>[2x]MKESAAAKFERQHMDSGNSPSSSSTYCNQMMRRRNMTQGRCKPVNTFVHESLVDVQNVCFQEKVTCKNGQGNCYKSNSSMHITDCRLTNGSRYP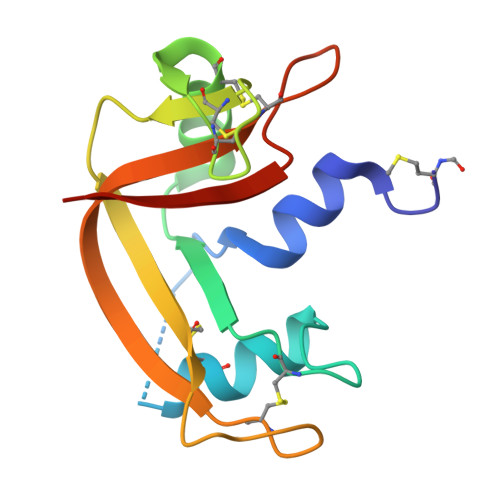NCAYRTSPKERHIIVACEGSPYVPVHFDASVEDST> M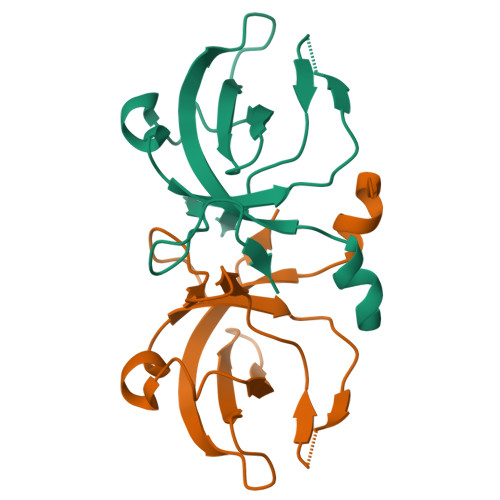YVKFDDFAKLDLRVGKIIEVKDHPNADKLYVVKVDLGDEVRTLVAGLKKYYKPEELLNRYVVVVANLEPKKLRGIGSQGMLLAADDGERVALLMPDKEVKLGAKVR>DTTPRRDAEYPPPELLEALKPLHDICLGKTGVTEEAIKKFSDEEIH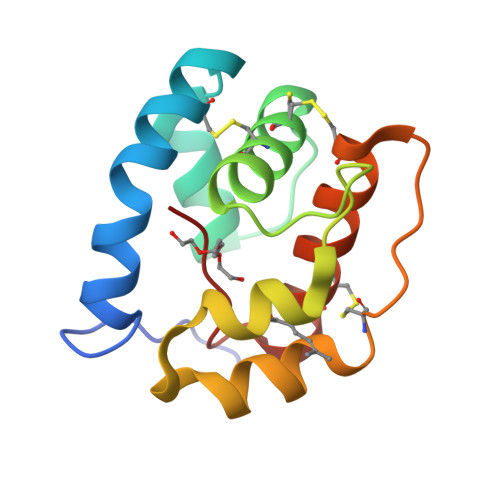EDEKLKCYMNCLFHEAKVVDDNGDVHLEKLHDSLPSSMHDIAMHMGKRCLYPEGETLCDKAFWLHKCWKQSDPKHYFLV[2x]> MTENILRKSDEEIQKEITARVKALESMLIEQGILTTSMIDRMAEIY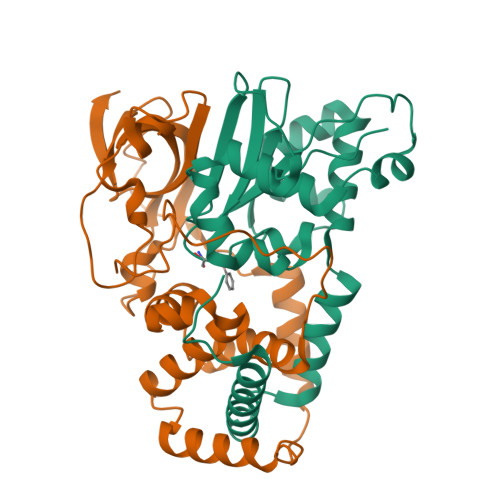ENEVGPHLGAKVVVKAWTDPEFKKRLLADGTEACKELGIGGLQGEDMMWVENTDEVHHVVVCTLCSCYPWPVLGLPPNWFKEPQYRSRVVREPRQLLKEEFGFEVPPSKEIKVWDSSSEMRFVVLPQRPAGTDGWSEEELATLVTRESMIGVEPAKAVHHHHHH;> MNGVYDVGGTDGLGPINRPADEPVFRAEWEKVAFAMFPATFRAGFMGLDEFRFGIEQMNPAEYLESPYYWHWIRTYIHHGVRTGKIDLEELERRTQYYRENPDAPLPEHEQKPELIEFVNQAVYGGLPASREVDRPPKFKEGDVVRFSTASPKGHARRARYVRGKTGTVVKHHGAYIYPDTAGNGLGECPEHLYTVRFTAQELWGPEGDPNSSVYYDCWEPYIELVDTKAAAA>MAHHHHHHSSGLEVLFQGPAAMGTSEKYAVVTGSNKGIGFETCKKLASQGIT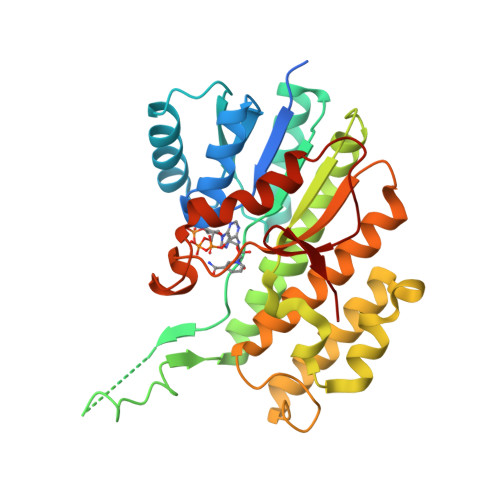VVLTARDEKRGLDALEKLKELGLSGKVLFHQLDVTDSSSVASLAEFVKKQFGRLDILVNNAGVNGVITDVEAVKKLNPAEDPADVDFSKIYKETYELAEECIQINYFGTKRTTDALLPLLQLSASPRIVNISSIMGQLKNIPSEWAKGILGDASNLTEDRLDEVINNFLKDFKEGSLAAKGWPPSFSAYIVSKVVVNAYTRILAKKYPNFKINCVCPGFAKTDLNHGLGLLTAEEAAENPVKLALLPDDGPSGLFFDRSEESSFE[2x]> XXXXXXXXXXXXXXXXXXXXXXXXXXXXXXXXXXXXXXXXXXXXXXXXXXXXXEMSQEESTRFYDQLNHHIFELVSSSDANERKGGILAIASLIGVEGGNATRIGRFANYLRNLLPSNDPVVMEMASKAIGRLAMAGDTFTAEYVEFEVKRALEWLGADRNEGRRHAAVLVLRELAISVPTFFFQQVQPFFDNIFVAVWDPKQAIREGAVAALRACLILTTQREPKEMQKPQWYRHTFEEAEKGFDETLAKEKGMNRDDRIHGALLILNELVRISSMEGERLREEMEEITQQQLVHDKYCKDLMGFGTKPRHITPFTSFQAVQPQQSNALVGLLGYSSHQGLMGFGTSPSPAKSTXXXXXXXXXXXXXXXXXXXXXXXXXRNSKNSLIQMTILNLLPRLAAFRPSAFTDTQYLQDTMNHVLSCVKKEKERTAAFQALGLLSVAVRSEFKVYLPRVLDIIRAALPPKDFAHKRQKAMQVDATVFTCISMLARAMGPGIQQDIKELLEPMLAVGLSPALTAVLYDLSRQIPQLKKDIQDGLLKMLSLVLMHKPLRHPGMPKGLAHQLASPGLTTLPEASDVGSITLALRTLGSFEFEGHSLTQFVRHCADHFLNSEHKEIRMEAARTCSRLLTPSIHLISGHAHVVSQTAVQVVADVLSKLLVVGITDPDPDIRYCVLASLDERFDAHLAQAENLQALFVALNDQVFEIRELAICTVGRLSSMNPAFVMPFLRKMLIQILTELEHSGIGRIKEQSARMLGHLVSNAPRLIRPYMEPILKALILKLKDPDPDPNPGVINNVLATIGELAQVSGLEMRKWVDELFIIIMDMLQDSSLLAKRQVALWTLGQLVASTGYVVEPYRKYPTLLEVLLNFLKTEQNQGTRREAIRVLGLLGALDPYKHKVNIGMIDQSRDASAVSLSESKSSQDSSDYSTSEMLVNMGNLPLDEFYPAVSMVALMRIFRDQSLSHHHTMVVQAITFIFKSLGLKCVQFLPQVMPTFLNVIRVCDGAIREFLFQQLGMLVSFVKSHIRPYMDEIVTLMREFWVMNTSIQSTIILLIEQIVVALGGEFKLYLPQLIPHMLRVFMHDNSPGRIVSIKLLAAIQLFGANLDDYLHLLLPPIVKLFDAPEAPLPSRKAALETVDRLTESLDFTDYASRIIHPIVRTLDQSPELRSTAMDTLSSLVFQLGKKYQIFIPMVNKVLVRHRINHQRYDVLICRIVKGYTLADEEEDPLIYQHRMLRSGQGDALASGPVETGPMKKLHVSTINLQKAWGAARRVSKDDWLEWLRRLSLELLKDSSSPSLRSCWALAQAYNPMARDLFNAAFVSCWSELNEDQQDELIRSIELALTSQDIAEVTQTLLNLAEFMEHSDKGPLPLRDDNGIVLLGERAAKCRAYAKALHYKELEFQKGPTPAILESLISINNKLQQPEAAAGVLEYAMKHFGELEIQATWYEKLHEWEDALVAYDKKMDTNKDDPELMLGRMRCLEALGEWGQLHQQCCEKWTLVNDETQAKMARMAAAAAWGLGQWDSMEEYTCMIPRDTHDGAFYRAVLALHQDLFSLAQQCIDKARDLLDAELTAMAGESYSRAYGAMVSCHMLSELEEVIQYKLVPERREIIRQIWWERLQGCQRIVEDWQKILMVRSLVVSPHEDMRTWLKYASLCGKSGRLALAHKTLVLLLGVDPSRQLDHPLPTVHPQVTYAYMKNMWKSARKIDAFQHMQHFVQTMQQQAQHAIATEDQQHKQELHKLMARCFLKLGEWQLNLQGINESTIPKVLQYYSAATEHDRSWYKAWHAWAVMNFEAVLHYKHQNQARDEKKKLRHASGANITNATTAATTAATATTTASTEGSNSESEAESTENSPTPSPLQKKVTEDLSKTLLMYTVPAVQGFFRSISLSRGNNLQDTLRVLTLWFDYGHWPDVNEALVEGVKAIQIDTWLQVIPQLIARIDTPRPLVGRLIHQLLTDIGRYHPQALIYPLTVASKSTTTARHNAANKILKNMCEHSNTLVQQAMMVSEELIRVAILWHEMWHEGLEEASRLYFGERNVKGMFEVLEPLHAMMERGPQTLKETSFNQAYGRDLMEAQEWCRKYMKSGNVKDLTQAWDLYYHVFRRISKQLPQLTSLELQYVSPKLLMCRDLELAVPGTYDPNQPIIRIQSIAPSLQVITSKQRPRKLTLMGSNGHEFVFLLKGHEDLRQDERVMQLFGLVNTLLANDPTSLRKNLSIQRYAVIPLSTNSGLIGWVPHCDTLHALIRDYREKKKILLNIEHRIMLRMAPDYDHLTLMQKVEVFEHAVNNTAGDDLAKLLWLKSPSSEVWFDRRTNYTRSLAVMSMVGYILGLGDRHPSNLMLDRLSGKILH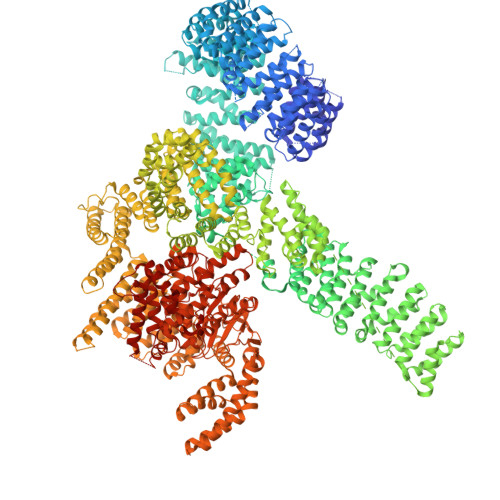IDFGDCFEVAMTREKFPEKIPFRLTRMLTNAMEVTGLDGNYRITCHTVMEVLREHKDSVMAVLEAFVYDPLLNWRLMDTNTKGNKRSRTRTDSYSAGQSVEILDGVELGEPAHKKTGTTVPESIHSFIGDGLVKPEALNKKAIQIINRVRDKLTGRDFSHDDTLDVPTQVELLIKQATSHENLCQCYIGWCPFW>[10x]MTTSASSHLNKGIKQVYMSLPQGEKVQAMYIWIDGTGEGLRCKTRTLDSEPKCVEELPEWNFDGSSTLQSEGSNSDMYLVPAAMFRDPFRKDPNKLVLCEVFKYNRRPAETNLRHTCKRIMDMVSNQHPWFGMEQEYTLMGTDGHPFGWPSNGFPGPQGPYYCGVGADRAYGRDIVEAHYRACLYAGVKIAGTNAEVMPAQWEFQIGPCEGISMGDHLWVARFILHRVCEDFGVIATFDPKPIPGNWNGAGCHTNFSTKAMREENGLKYIEEAIEKLSKRHQYHIRAYDPKGGLDNARRLTGFHETSNINDFSAGVANRSASIRIPRTVGQEKKGYFEDRRPSANCDPFSVTEALIRTCLLNETGDEPFQYKN

Here we report the use of “Build and Retrieve” to define the composition of a raw human brain microsomal lysate. From this sample, we simultaneously identify and solve cryo-EM structures of five different brain enzymes whose functions affect neurotransmitter recycling, iron metabolism, glycolysis, axonal development, energy homeostasis, and retinoic acid biosynthesis. Collectively, the BaR approach was then used to reveal enzyme identities and solve cryo-EM structures of these brain enzymes with resolutions ranging between 2.69 and 3.40 Å. These enzymes were identified as glutamine synthetase (GS), ferritin (FT), dihydropyrimidinase-related protein 2 (DPYSL2), glyceraldehyde 3-phosphate dehydrogenase (GAPDH), and retinaldehyde dehydrogenase 1 (ALDH1A1). Interestingly, malfunction of these important proteins has been directly linked to several neurodegenerative disorders, such as Alzheimer’s, Huntington’s, and Parkinson’s diseases.

GS is a glutamine synthesizing enzyme engaged in the recycling of synaptically released glutamate and γ-aminobutyric acid (GABA) and the detoxification of ammonia. Subsequently, we were able to identify this protein as the GS enzyme and resolve its structure to a resolution of 2.73 Å. Human GS assembles as an oligomer of 10 subunits, creating a dimer of pentamers. The two pentamers stack against each other to form two layers. Each subunit of GS consists of a small N-terminal domain (residues 2–102) and a large C-terminal domain (residues 114–372). Based on the structure, the N-terminal domain contributes to subunit–subunit interactions within each layer of the pentamer, whereas the C-terminal domain participates in forming the catalytic site for substrate binding. However, the loop residues (residues 149–157) of the C-terminal domain of each GS subunit are responsible for securing interactions between two pentameric layers. Within the active site of the C-terminal catalytic domain of each subunit of human GS, we observed a bound Mn2+ ion, which is anchored by residues E134, H253, and E338. This catalytic site also contains several other positively charged residues, including R299, R319, R324, R340, and R341, that contribute to substrate binding. (i) In two unrelated cases, newborns were found to have congenital glutamine deficiency consisting of two-point mutations (R324C and R341C) on the GS enzyme.> MSILNDYKRKTEGSVFWAQRARSVMPDGVTADTRAFDPHGLFISDAQGVHKTDVDGNVYLDFFGGHGALVLGHGHPRVNAAIAEALSHGVQYAASHPLEVRWAERIVAAFPSIRKLRFTGSGTETTLLALRVARAFTGRRMILRFEGHYHGWHDFSASGYNSHFDGQPAPGVLPETTANTLLIRPDDIEGMREVFANHGSDIAAFIAEPVGSHFGVTPVSDSFLREGAELARQYGALFILDEVISGFRVGNHGMQALLDVQPDLTCLAKASAGGLPGGILGGREDVMGVLSRGSDRKVLHQGTFTGNPITAAAAIAAIDTILEDDVCAKINDLGQFAREAMNHLFARKGLNWLAYGRFSGFHLMPGLPPNTTDTGSITRAEVARPDVKMIAAMRMALILEGVDIGGRGSVFLS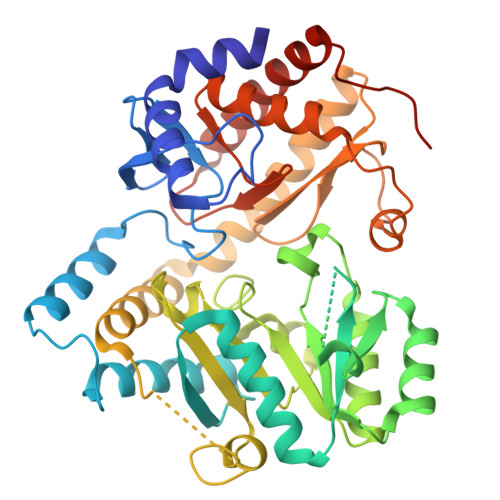AQHEREHVEHLVTTFDRVLDRLADENLLSWQGTNLSGNQS> MATINNVTDLAIAAIQWSDRQDLTQELLMLFI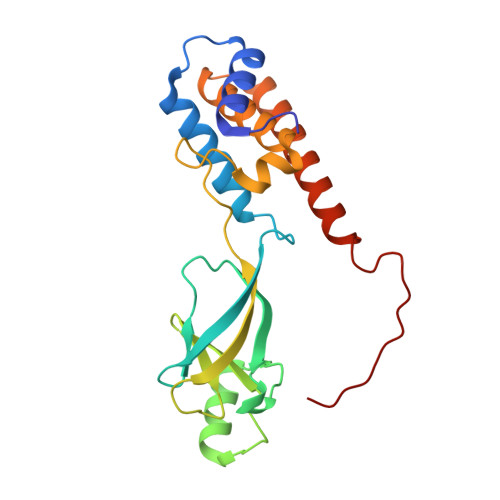GNTTDRLNRLLRVRENEHFETLMAFGGGIEIPEHFVALRSITGDSLIGGRTLQYITQDIFTHYVNYNYQPQGVTYYTRLGNFWRVFPVVPDGAPFIVNYWTVLPELSLANPTTWALTKYPQIYLYGVLEQIYLYTMDEARSQFWGQKLERAVMELQNEENAADFASTRLAIKDIER> MSLNGNGSIELKGTVEEVWSKLMDPSILSKCIMGCKSLELIGEDKYKADLQIGIAAVKGKYDAIIEVTDIKPPYHYKL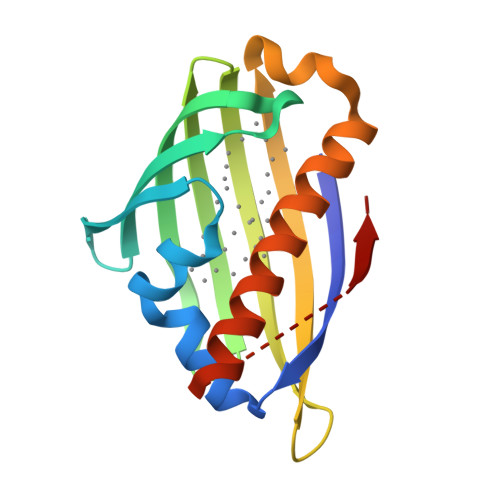LVNGEGGPGFVNAEGVIDLTPINDECTQLTYTYSAEVGGKVAAIGQRMLGGVAKLLISDFFKKIQKEIAKSKQEASEGHHHHHH> MAGLNDIFEAQKIEWHELEVLFQGPMSPDVVLVNGGEPPNPLIPTGTNDSNGGRIIDRLFAGLMSYDAVGKPSLEVAQSIESADNVNYRITVKPGWKFTDGSPVTAHSFVDAWNYGALSTNAQLQQHFFSPIEGFDDVAGAPGDKSRTTMSGLRVVNDLEFTVRLKAPTIDFTLRLGHSSFYPLPDSAFRDMAAFGRNPIGNGPYKLADGPAGPAWEHNVRIDLVPNPD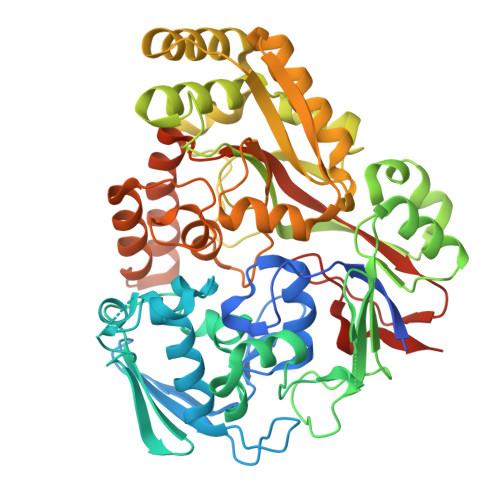YHGNRKPRNKGLRFEFYANLDTAYADLLSGNLDVLDTIPPSALTVYQRDLGDHATSGPAAINQTLDTPLRLPHFGGEEGRLRRLALSAAINRPQICQQIFAGTRSPARDFTARSLPGFDPNLPGNEVLDYDPQRARRLWAQADAISPWSGRYAIAYNADAGHRDWVDAVANSIKNVLGIDAVAAPQPTFAGFRTQITNRAIDSAFRAGWRGDYPSMIEFLAPLFTAGAGSNDVGYINPEFDAALAAAEAAPTLTESHELVNDAQRILFHDMPVVPLWDYISVVGWSSQVSNVTVTWNGLPDYENIVKAENLYFQGGHHHHHHHH As part of investigations into the C-nucleoside formycin A (8-aza-9-deazaadenosine) biosynthetic gene cluster from Streptomyces kaniharaensis, we have characterised a pyridoxal 5′-phosphate (PLP) dependent aminotransferase (ForI) that aminates a pathway intermediate. ForI is a PLP-dependent enzyme from the biosynthetic pathway of the C-nucleoside antibiotic formycin. ForI possesses the mixed β-sheet and three-stranded antiparallel β-sheet insertion characteristic of the PLP dependent aspartic aminotransferase family. The predicted active site of ForI comprises residues from two monomers, indicating the dimer to be the functional unit.

The enzyme purifies with bound PLP and exists as a dimer (ESI†). Residues 3 to 417 were located experimentally; the missing nine residues we assume to be conformationally flexible. Electron density shows that PLP forms a Schiff base (internal aldimine) with the active site Lys 262. The dimer arises from crystal symmetry. The resolution of the structure allows for visualisation of extensive hydration at the active site and water–PLP hydrogen bonds. PLP makes multiple contacts with the protein, broadly similar to those described for the GSAAT structure. The equivalent residues in ForI adopt a different arrangement creating a cavity (pocket) adjacent to PLP. The substitution of Met 248 in GSAAT by Gly 238 in ForI also leads to a more open active site (ESI†). In ForI, Trp 206 and Arg 207 which are not present in GSAAT, only partially fill the pocket. The consequence of these changes is that the pocket adjacent to the co-factor is larger in ForI.

> AMITEKSAALYARAVEVMPGGNSRTAVYSSPYPVYVRSGSGARVTDVDGVERIDFLNNSTTLIHGHAHPEMVEAIAAAVGHGTSFGMPTPVEVEYAEALSARNETFEHVRFTSSGTEAVMMAVQAARAYTERPKIAKIAGAYHGAYDAVAVNNDGSGNLISHAVTGNPEGVVANTVVIPFNDPEGSLEVLRRHADDLACVLIDPVPWRIGLLPASKEWLDALREFCDASGAVLISDEVGSYRVGYHGAMQLLGAEADITVMGKVIAAGMPIGAVAGRRRFMSVFDPSKGKPALPHSGSYNANPVSMSSGIASLRLLTPQAHERIGQLGEQARGSMRTALGEAGLDWEVNGLGSLFRVVANSAPAGYDSAAAAMKALYWKLLENGIHIGDSGLGCISTPMGEEEIAEYAVAFAKSLGQVLAEGRA> MQSVGGDSSADRLFPPQWICCDIRYLDVSILGKFAVVMADPPWDIHMELPYGTLTDDEMRRLNIPVLQDDGFLFLWVTGRAMELGRECLNLWGYERVDEIIWVKTNQLQRIIRTGRTGHWLNHGKEHCLVGVKGNPQGFNQGLDCDVIVAEVRSTSHKPDEIYGMIERLSPGTRKIELFGRPHNVQPNWITLGNQLDGIHLLDPDVVARFKQRYPDGIISKPKNL;> GSGQSLNPHNDYCQHFV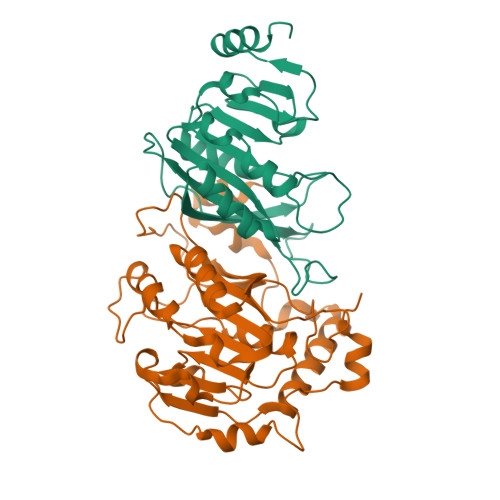DTGHRPQNFIRDVGLADRFEEYPKLRELIRLKDELIAKSNTPPMYLQADIEAFDIRELTPKFDVILLEPPLEEYYRETGITANEKCWTWDDIMKLEIDEIAAPRSFIFLWCGSGEGLDLGRVCLRKWGYRRCEDICWIKTNKNNPGKTKTLDPKAVFQRTKEHCLMGIKGTVKPSTDGDFIHANVDIDLIITEEPEIGNIEKPVEIFHIIEHFCLGRRRLHLFGRDSTIRPGWLTVGPTLTNSNYNAETYASYFSAPNSYLTGCTEEIERLRPKSPPPKSKSDRGGGAPRGGGRGGTSAGRGRERNRSNFRGERGGFRGGRGGAHRGGFPPR>[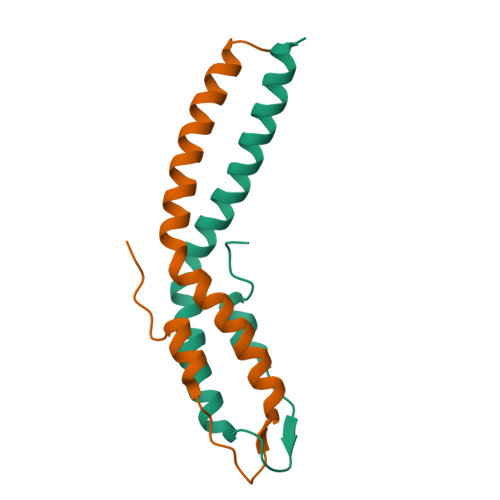2x]MSDVSLKLSAKDIYEKDFEKTMARGYRREEVDAFLDDIIADYQKMADMNNEVVKLSEENHKLKKELEELRLRVAT>[2x]MASWSHPQFEKGAVTSLYKKAGFQKVTFKEETYQLEGKALKVGDKAPDVKLVNGDLQEVNLLKQGVRFQVVSALPSL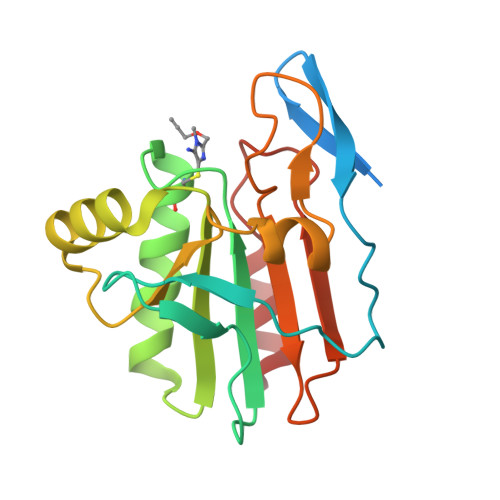TGSVCLLQAKHFNEQTGKLPSVSFSVISMDLPFSQGQIAGAEGIKDLRILSDFRYKAFGENYGVLLGKGSLQGLLARSVFVLDDKGVVIYKEIVQNILEEPNYEALLKVLK> KEQTSFNNPEPMTGFEHTVTFDFQGTKMVIPYGYLARYTQDNATKWLS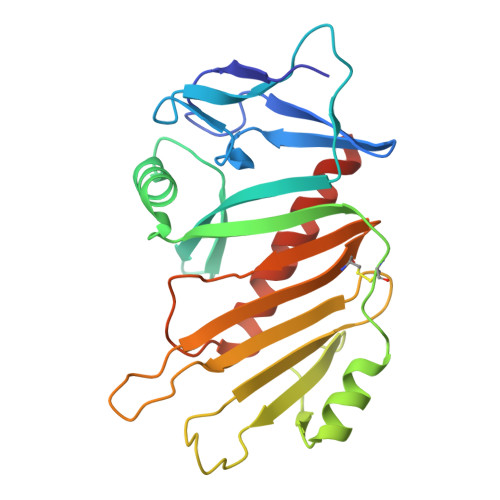DTPGQDAYSINLIEISVYYKKTDQGWVLEPYNQQNKAHFIQFLRDGLDSVDDIVIRKDACSLSTTMGERLLTYGVKKMPSAYPEYEAYEDKRHIPENPYFHEFYYIKKGENPAIITHRNNRINQTEEDSYSTSVGSCINGFTVQYYPFIREKQQLTQQELVGYHQQVEQLVQSFVNNSNKKLE> LSKYGGECSKEHNTCTYRKDGKD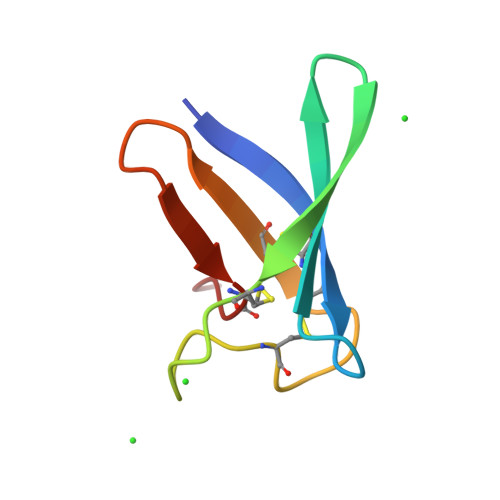HIVKCPSADNKKCKTDRHHCEYDSYDRKVDCQTPV>MNDRDFMRYSRQILLDDIALDGQQKLLDSQVLIIGLGGLGTPAALYLAGAGVGTLVLADDDDVHLSNLQRQILFTTEDIDRPKSQVSQQRLTQLNPDIQLTALQQRLTGEALKDAVARADVVLDCTDNMATRQEINAACVALNTPLITASAVGFGGQLMVLTPPWEQGCYRCLWPDNQEPERNCRTAGVVGPVVGVMGTLQALEAIKLLSGIETPAGELRLFDGKSSQWRSLALRRASGCPVCGGSNADPV[2x];>MQILFNDQAMQCAAGQTVHELLEQLDQRQAGAALAINQQIVPREQWAQHIVQD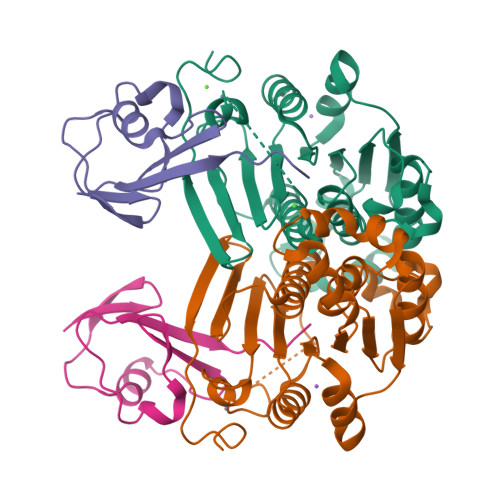GDQILLFQVIAGG[2x]>[3x]MKKLLTVMTMAVLTAGTLLLPAQSVTPAAHAVQISN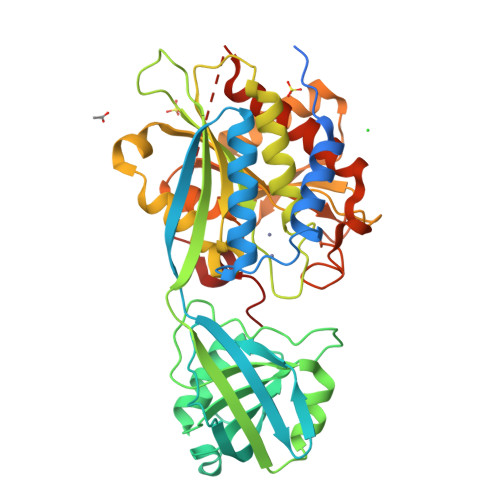SERELPFKAKHAYSTISQLSEAIGPRIAGTAAEKKSALLIASSMRKLKLDVKVQRFNIPDRLEGTLSSAGRDILLQAASGSAPTEEQGLTAPLYNAGLGYQKDFTADAKGKIALISRGDLTYYEKAKNAEAAGAKAVIIYNNKESLVPMTPNLSGNKVGIPVVGIKKEDGEALTQQKEATLKLKAFTNQTSQNIIGIKKPKNIKHPDIVYVTAHYDSVPFSPGANDNGSGTSVMLEMARVLKSVPSDKEIRFIAFGAEELGLLGSSHYVDHLSEKELKRSEVNFNLDMVGTSWEKASELYVNTLDGQSNYVWESSRTAAEKIGFDSLSLTQGGSSDHVPFHEAGIDSANFIWGDPETEEVEPWYHTPEDSIEHISKERLQQAGDLVTAAVYEAVKKEKKPKTIKKQMKAKASDIFEDIK>[2x]GGGWLEAEKKGAPQKDSTGGVLEESNKIEPSLHSLQKFVPTDYASYTQEHYRFAGKEI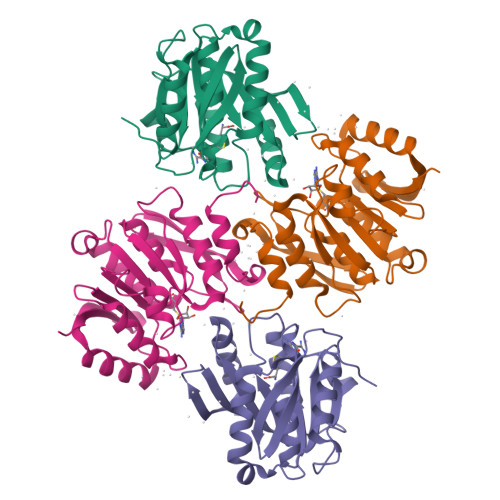VIQESIESYGAVVWPGAMALCQYLEEHAEELNFQDAKILEIGAGPGLVSIVASILGAQVTATDLPDVLGNLQYNLLKNTLQCTAHLPEVKELVWGEDLDKNFPKSAFYYDYVLASDVVYHHYFLDKLLTTMVYLSQPGTVLLWANKFRFSTDYEFLDKFKQVFDTTLLAEYPESSVKLFKGILKWD Repulsive guidance molecules (RGMs) are cell surface proteins that control processes ranging from brain development to iron metabolism. RGMs can bind to the cell guidance receptor Neogenin (NEO1) and act as coreceptors for the bone morphogenetic proteins (BMPs). Structural analysis of RGMs and their complexes with NEO1 and BMP2 revealed a common RGM architecture comprising an N-terminal domain (RGMND) essential for BMP binding and a C-terminal domain (RGMCD) sufficient for NEO1 binding. Here, we determined high-resolution structures of all three human RGMs in complex with the BMP ligand growth differentiation factor 5 (GDF5) and the ternary complex of GDF5 with RGM and NEO1.

To test this hypothesis, we determined the structure of the ternary complex between the two membrane proximal NEO1 fibronectin-type III domains (NEO1FN56), RGMBECD and GDF5 to 5.5 Å resolution. In the complex, the GDF5 dimer binds to two RGMB ectodomains in a similar arrangement to that in the binary RGMBND–GDF5 complex. RGMBND is connected to the RGMB C-terminal domain (RGMBCD) via a flexible linker (∼12 residues), as suggested by its fragmentary electron density. RGMBCD is sandwiched between GDF5 and NEO1. A hydrophobic face of RGMBCD (Phe162–Phe166, Arg172, Tyr268–Glu270, Phe281, Ala292) interacts with a hydrophobic region of GDF5 (Ile419–Leu422, Val485–Tyr487, Leu477–Ile479). However, this interaction is likely to play a minor role in the RGMB–GDF5 interactions, as RGMBND is sufficient to bind to GDF5 with high affinity. RGMBCD uses an opposite face of the β-sandwich to bind NEO1, resembling the main interface previously observed in the binary NEO1–RGMB complex. The 2:2:2 NEO1–RGMB–GDF5 architecture is compatible with a potential arrangement of RGMs, NEO1, and GDF5 on the cell surface. C termini of RGMB and NEO1 point in the same direction and could be accommodated on the surface of one cell to control downstream signaling. In summary, our structural analysis of the ternary NEO1–RGMB–GDF5 complex combined with cellular assays reveal the modular architecture of RGMB where its N-terminal domain acts as a robust inhibitor of GDF5 signaling, whereas its C-terminal domain interacts with NEO1.

>MKRQGKRPSKNLKARCSRKALHVNFKDMGWDDWIIAPLEYEAFHCEGLCEFPLRSHLEPTNHAVIQTLMNSMDPESTPPTCCVPTRLSPISILFIDSANNVVYKQYEDMVVESCGCR[6x];>[18x]ETGQCRIQKCTTDFVSLTSHLNSAVDGFDSEFCKALRAYAGCTQRTSKACRGNLVYHSAVLGISDLMSQRNCSKDGPTSSTNPEVTHDPCNYHSHAGAREHRRGDQNPPSYLFCGLFGDPHLRTFKDNFQTCKVEGAWPLIDNNYLSVQVTNVPVVPGSSATATNKITIIFKAHHGCTDQKVYQAVTDDLPAAFVDGTTSGGDSDAKSLRIVERESGHYVEMHARYIGTTVFVRQVGRYLTLAIRMPEDLAMSYEESQDLQLCVNGCPLSERIDDGQGQVSAILGHSLPRTSLVQAWPGYTLETANTQCHEKMPVKDIYFQSCVFDLLTTGDANFTAAAHSALEDVEALHPRKERWHIFPSSGTKHHHHHH;>[6x]ETGTPMMPPVGVQASILSHDTIRITWADNSLPKHQKITDSRYYTVRWKTNIPANTKYKNANATTLSYLVTGLKPNTLYEFSVMVTKGRRSSTWSMTAHGATFELVPTSPPKDVTVVSKEGKPRTIIVNWQPPSEANGKITGYIIYYSTDVNAEIHDWVIEPVVGNRLTHQIQELTLDTPYYFKIQARNSKGMGPMSEAVQFRTPKALGSAGKGSRLPDLGSDYKPPMSGSNSPHGSPTSPLDSNGTKHHHHHH6-[[4-[(3-methylsulfonylphenyl)methylamino]-5-(trifluoromethyl)pyrimidin-2-yl]amino]-3,4-dihydro-1~{H}-quinolin-2-one 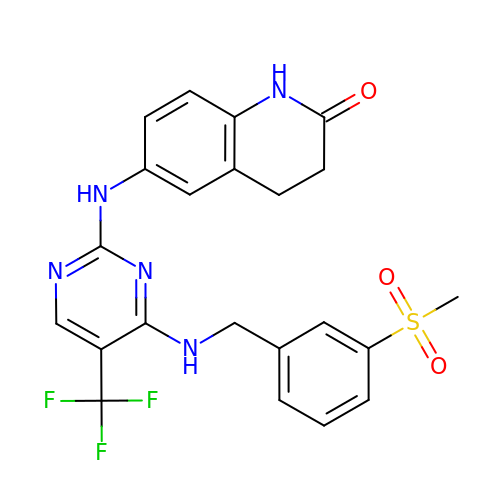| C22 H20 F3 N5 O3 S | HESLKTSGTIBHJU-UHFFFAOYSA-N> GSIDESRIGDVHKHTGRNCGRKF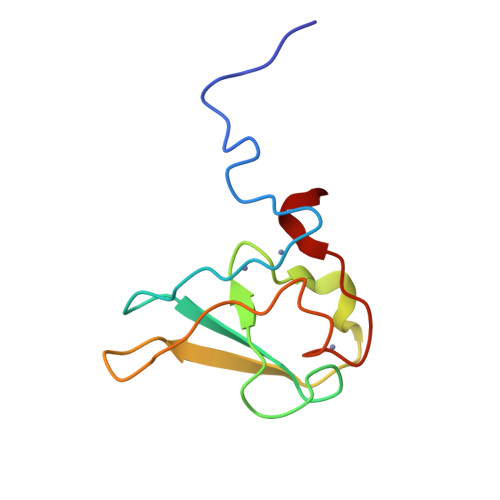KIGEPLYRCHECGCDDTCVLCIHCFNPKDHVNHHVCTDICTEFTSGICDCGDEEAWNSPLHCKAEEQ>[2x]STAGKVIKCKAAVLWEEKKPFSIEEVEVAPPKAH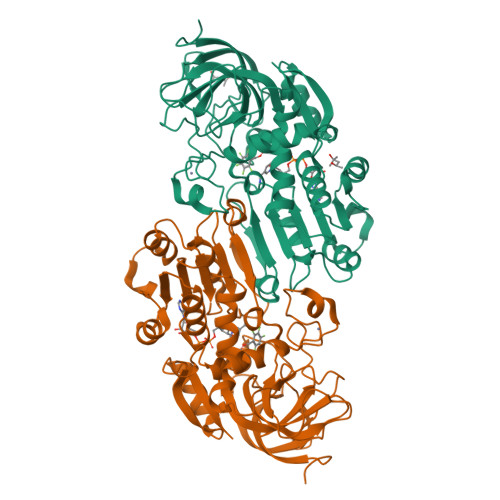EVRIKMVATGICRSDDHVVSGTLVTPLPVIAGHEAAGIVESIGEGVTTVRPGDKVIPLFTPQCGKCRVCKHPEGNFCLKNDLSMPRGTMQDGTSRFTCRGKPIHHFLGTSTFSQYTVVDEISVAKIDAASPLEKVCLIGCGFSTGYGSAVKVAKVTQGSTCAVFGLGGVGLSVIMGCKAAGAARILGVDINKDKFAKAKEVGATECVNPQDYKKPIQEVLTEMSNGGVDFSFEVIGRLDTMVTALSCCQEAYGVSVIVGVPPDSQNLSMNPMLLLSGRTWKGAIFGGFKSKDSVPKLVADFMAKKFALDPLITHVLPFEKINEGFDLLRSGESIRTILTF>DPIHYDKITEEINKAIDDAIAAIEQSETIDPMKVPDHADKFERHVGILDFKGELAMRNIEARGLKQMKRQGDANVKGEEGIVKAHLLIGVHDDIVSMEYDLAYKLGDLHPTTHVISDIQDFVVALSLEIPDEGNITMT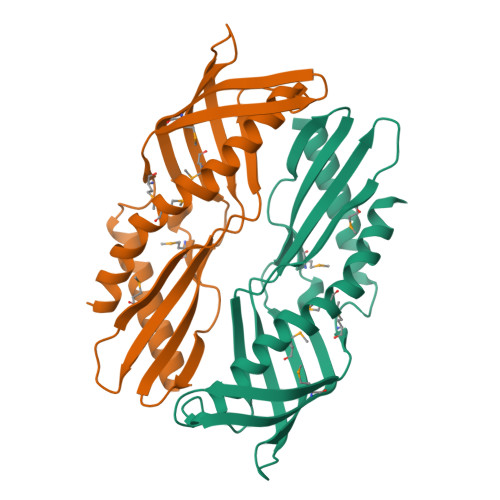SFEVRQFANVVNHIGGLSILDPIFGVLSDVLTAIFQDTVRKEMTKVLAPAFKRELEKN[2x]>[8x]SMADRGDSGDSDFVVVANRLPIDLERAPDGTTSWKRSPGGLVTALEPLLRRRRGAWIGWPGIPDSDEDPIVDGDLVLYPVRLSADDVAQYYEGFSNATLWPLYHDVIVKPIYNRQWWERYVEVNRRFAEATSRAAARGATVWVQDYQLQLVPKMLRELRPDLTIGFFLHIPFPPVEL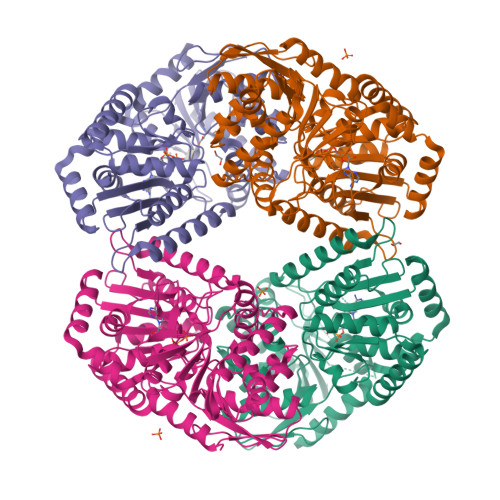FMQLPWRTEITDGLLGADLVGFHLPGGAQNFLFLARRLVGANTSRASVGVRSKFGEVQIGSRTVKVGAFPISIDSADLDRQARQRSIRQRARQIRAELGNPRRILLGVDRLDYTKGIDVRLQAFAELLAEGRVNREDTVFVQLATPSRERVEAYRLLRDDIERQVGHINGEYGEVGHPVVHYLHRPVPREELIAFFVAADVMLVTPLRDGMNLVAKEYVACRSDLGGALVLSEFTGAAAELGQAYLVNPHNLDHVKDTMVAALNQTPEEGRRRMRALRRQVLAHDVDLWARSFLDALASTRTGDADAVPV endosulfan | C9 H6 Cl6 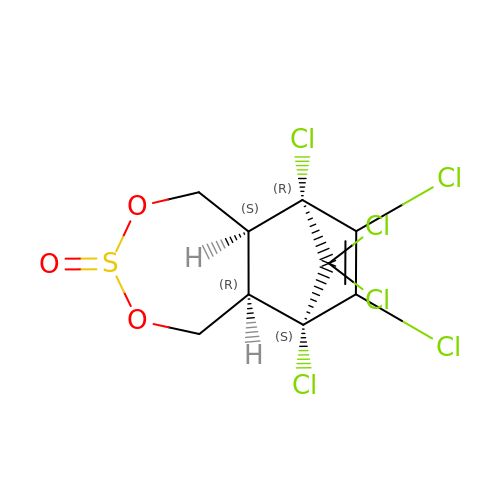O3 S | RDYMFSUJUZBWLH-BEJSPLBDSA-N> DSDS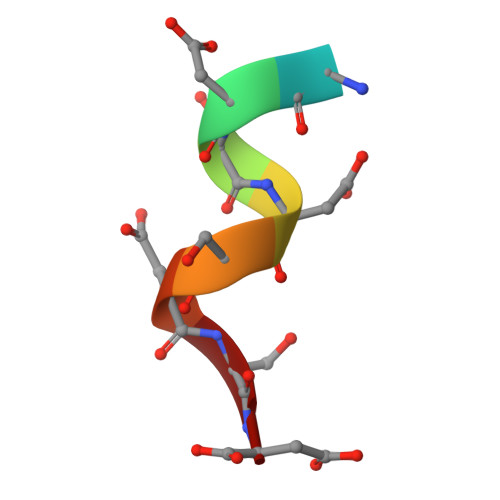DSDSD>[2x]GSNRSLIVTTLLEEPFVMFRKSDRTLYGNDRFEGYCIDLLKELAHILGFSYEIRLVEDGKYGAQDD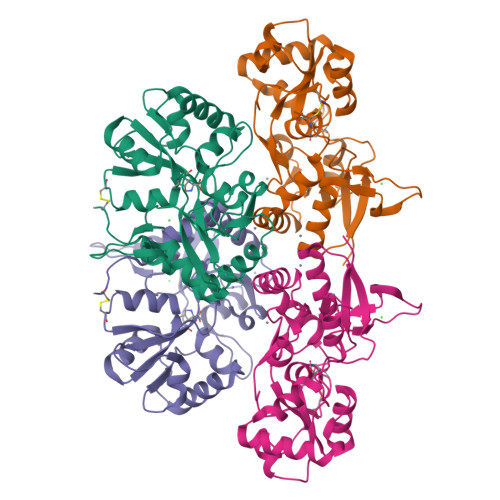KGQWNGMVKELIDHKADLAVAPLTITHVREKAIDFSKPFMTLGVSILYRKGTPIDSADDLAKQTKIEYGAVKDGATMTFFKKSKISTFEKMWAFMSSKPSALVKNNEEGIQRTLTADYALLMESTTIEYITQRNCNLTQIGGLIDSKGYGIGTPMGSPYRDKITIAILQLQEEDKLHIMKEKWWRGSGCPE>MGSSHHHHHHSSGLQGTENLYFQSHMSELIVNVINGPNLGRLGRREPAVYGGTTHDELVALIEREAAELGLKAVVRQSDSEAQLLDWIHQAADAAEPVILNAGGLTHTSVALRDACAE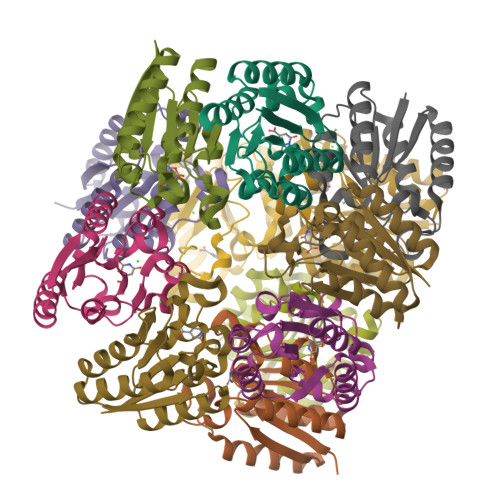LSAPLIEVHISNVHAREEFRRHSYLSPIATGVIVGLGIQGYLLALRYLAEHVGT[24x]> ETFSGGCLFDEPYSTCGYSQSEGDDFNWEQVNTLTKPTSDPWMPSGSFMLVNASGRPEGQRAHLLLPQLKENDTHCIDFHYFVSSKSNSPPGLLNVYVKVNNGPLGNPIWNISGDPTRTWNRAELAISTFWPNFYQVIFEVITSGHQGYLAIDEVKVLGHPCTRTPHFLRIQNVEVNAGQFATFQCSAIGRTVAGDRLWLQGIDVRDAPLKEIKVTSSRRFIASFNVVNTTKRD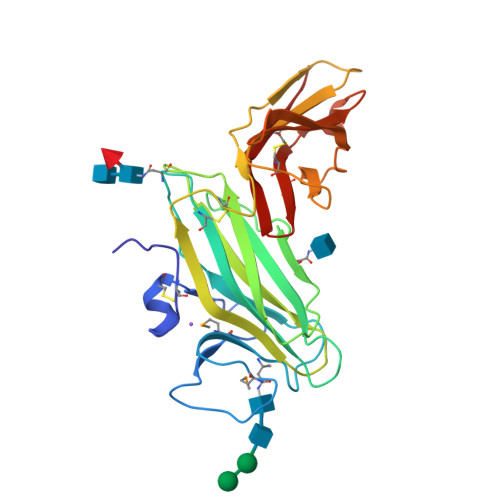AGKYRCMIRTEGGVGISNYAELVVK Salmonella enterica serovar Typhimurium (S. Typhimurium), a gram-negative bacterium responsible for innumerable cases of acute gastroenteritis worldwide, utilizes two T3SSs, encoded within its pathogenicity islands 1 (SPI-1) and 2 (SPI-2), to invade cells and establish an intracellular replicative niche. The core component of this machine is the envelope-associated needle complex, which consists of a multiring base, an inner rod, and a needle filament extension that protrudes several nanometers from the bacterial surface. The entire structure is traversed by an approximately 2-nm channel that serves as a conduit for the T3SS protein substrates as they pass through the bacterial envelope. Furthermore, four residues at the end of the C-terminal α-helix, three charged (K66, D70, and R80) and one polar uncharged (Q77), form the lumen of the channel and create an electrostatic surface potential of alternating charges, which spiral upwardly about the needle, a feature that has been proposed to be important for substrate translocation.

In contrast, and as previously reported for the cryo-EM structure of isolated filaments, our structure differs from the SSNMR structure of in vitro assembled filaments. Even the closest structure of all 10 SSNMR models reported shows a difference in the twist (63.35° in our model versus 64.00° in the SSNMR model), which although relatively minor, leads to accumulating differences that ultimately results in noticeable variance in subunit packing. Consequently, the overall fitting of the two structures is poor. The reasons for the observed differences between the cryo-EM and the SSNMR structures could be due to structural differences resulting from the different assembly mechanisms (i.e., in vitro versus in vivo) or differences strictly related to the methodologies utilized to determine the structures (i.e., cryo-EM versus SSNMR). To clarify this issue, we solved the cryo-EM structure of in vitro polymerized PrgI needle filaments. We found that the structures of in vitro polymerized needle filaments is virtually identical to the structure of in vivo assembled filaments attached to the base structure, exhibiting equivalent helical twist and rise. These results indicate that the differences between the cryo-EM structures of in vivo assembled filaments and the SSNMR structure of in vitro assembled needle filaments is due to differences in the experimental approaches utilized to solve the different structures rather than differences resulting from the assembly mechanisms.

>[18x]GSHMATPWSGYLDDVSAKFDTGVDNLQTQVTEALDKLAAKPSDPALLAAYQSKLSEYNLYRNAQSNTVKVFKDIDAAIIQNFR> TVDDILEQVGESGWFQKQAFLILCLLSAAFAPICVGIVFLGFTPDHHCQSPGVAELSQRCGWSPAEELNYTVPGLGPAGEAFLGQCRRYEVDWNQSALSCVDPLASLATNRSHLPLGPCQDGWVYDTPGSSIVTEFNLVCADSWKLDLFQSCLNAGFLFGSLGVGYFADRFGRKLCLLGTVLVNAVSGVLMAFSPNYMSMLLFRLLQGLVSKGNWMAGYTLITEFVGSGSRRTVAIMYQMAFTVGLVALTGLAYALPHWRWLQLAVSLPTFLFLLYYWCVPESPRWLLSQKRNTEAIKIMDHIAQKNGKLPPADLKMLSLEEDVTEKLSPSFADLFRTPRLRKRTFILMYLWFTDSVLYQGLILHMGATSGNLYLDFLYSALVEIPGAFIALITIDRVGRIYPMAMSNLLAGAACLVMIFISPDLHWLNIIIMCVGRMGITIAIQMICLVNAELYPTFVRNLGVMVCSSLCDIGGIITPFIVFRLREVWQALPLILFAVLGLLAAGVTLLLPE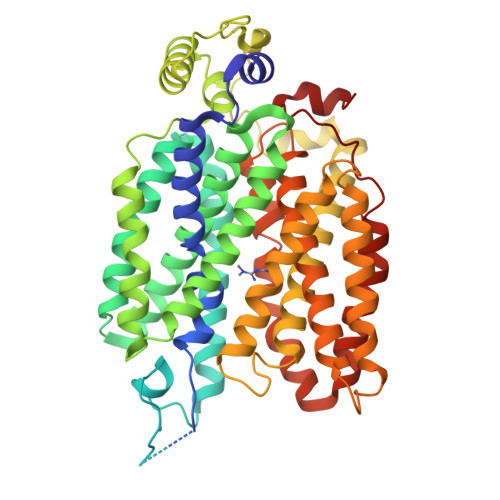TKGVALPETMKDAENLG>[12x]MVVIGEKFPEVEVKTTHGRIKLPDYFTKQGKWFILFSHPADFTPVCTTEFYGMQKRVEEFRKLGVEPIGLSVDQVEDHSAWIEWIKDNLSVEIDFPVIADDRG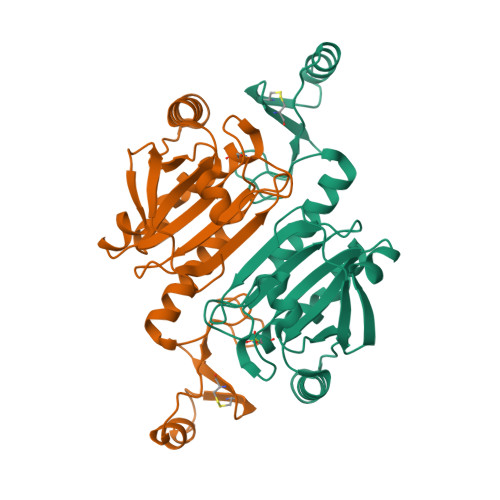ELAEKLGMIPSGATITARAVFVVDDKGIIRAIVYYPAEVGRDWDEILRLVKALKISTEKGVALPHKWPNNELIGDKVIVPPASTIEEKKQREEAKAKGEIECYDSWFCYKKLE> GSHMTKYKYTVEESERFNKHGIDLTVYGQVDPSATVVRVSVERGHFQEFFNVRSSYTFYVVSGQGVFYLNSEAVPAGATDLITVPPNTRIHYFGSMEMVLTVAPAFNEQDERHVRFISESESPY

In pacidamycin 3, biosynthesis the 3′‐deoxy moiety is mediated by Pac13, an enzyme found to catalyze the key dehydration of uridine‐5′‐aldehyde 1 to form 3′‐deoxy‐3′,4′‐didehydrouridine‐5′‐aldehyde 2. In stark contrast to most characterised dehydratases, Pac13 is small (121 aa), monomeric, co‐factor independent and utilises a non‐activated nucleoside, rather than a free monosaccharide, as a substrate. Pac13 is the only monomeric, metal‐free cupin dehydratase characterised to date. We demonstrate here that the reaction most likely proceeds via an E1Cb mechanism, with H42 acting as an active site base, however, unlike many other dehydratases, no metal or cofactor is required for activity.

Mutants E108Q, K16R, H42Q, Y55F and Y89F were produced and purified, affording diffracting crystals of the same morphology and space group as wt Pac13, which raised our confidence that the mutants folded correctly and that the effects seen are specific to interactions with each mutated residue rather than global effects on protein folding and structure. The kinetic measurements for the activity of Y55F and K16R demonstrated lower affinity and catalytic efficiency than wt Pac13. Finally, the significant loss of activity with mutants Y89F and Y55F is consistent with their proposed involvement in stabilizing the oxyanion and underlines their important role for catalysis. Similarly, on examining the Y89F–uridine complex and Y55F–uridine complex structures, we observed a high degree of similarity with the wt enzyme. Although there are subtle shifts in the position of both the ribose and uracil rings, of the substrate, and in the orientation of the 5′ functionality, these changes are small and consistent with our hypothesis that decreased catalytic efficiency of these mutants is largely due to inability of the phenyl mutants to stabilize the transient 5′ oxo‐anion that forms during catalysis, rather than having a major effect on binding competency.>ARPRVLTGDRPTGALHLGHLAGSLQNRVRLQDEAELFVLLADVQALTDHFDRPEQVRENVLAVALDYLAAGLDPQKTTCVVQSAVPELAELTVYFLNLVTVSHLRQNPTVKAEIAQKGYGERVPAGFFVYPVSQAADIA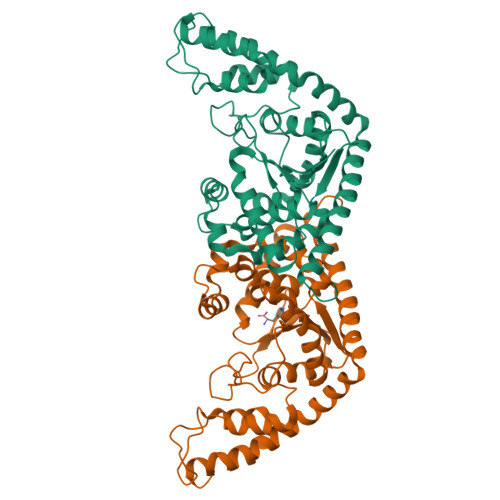AFGATLVPVGDDQLPMLEQTREIVRRFNALYAPVLAEPQAQLSRVPRLPGLDGQAKMSKSLGNAIALGDSADEVARKVMGMYTDPGHLRASDPGRVEGNPVFTFLDAFDPDPARVQALKDQYRAGGLGDVKVKKHLIDVLNGVLAPIRTRRAEYERDPDAVLRFVTEGTARGREVAAQTLGQVRRAMRLFGH[3x]>[2x]MDGTAEKQRDSLASRYKASTDYAKDAEGLTAPYVSQDPQETAALVRALDDAAKKGKKSGGFSVKKTRYAVASSPTGAEVDSWRFNDWDYKKPDLPTYARGLFTTRTQHGVPEIAVRGYDKFFNIDETRDTAWSAIRERTKGPYELTLKENGCIIFISGLEDGTLLVCSKHSTGDRSDVALSHSSAGEKHLEAQLERIGKTKEELARELRKRNATAVAELCDDSFEEHILAYGPDKAG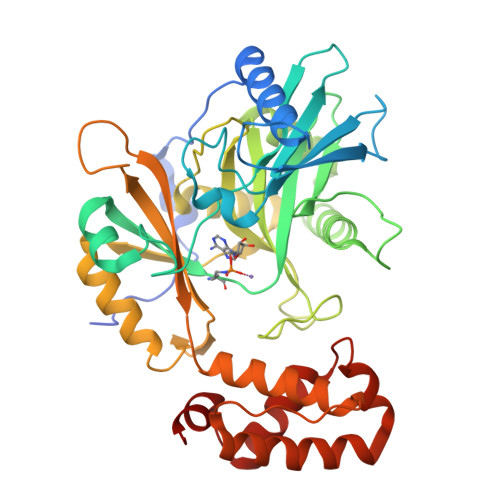LYLHGINLNIPEFITYPSPLVQKFAEDWGFRKTGLIIIDNIDDVKAFLEEVAETGAHDGRDVEGFVIRCKKSTNPGVGPYHDWFFKYKFEEPYLMYRQWRECTKALISGKQPKIKKHVKITEEYLLYARKRLAADPKLAKLYNQNHGIIKLRNDFLEYKNMKGTDAANLE FELODIPINE | C18 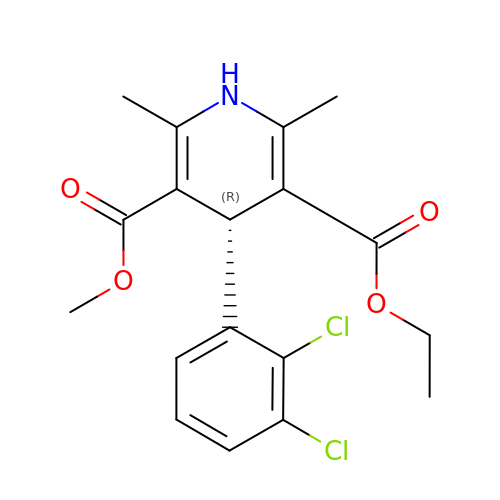H19 Cl2 N O4 | RZTAMFZIAATZDJ-OAHLLOKOSA-N>MLEYPIGTPQNLA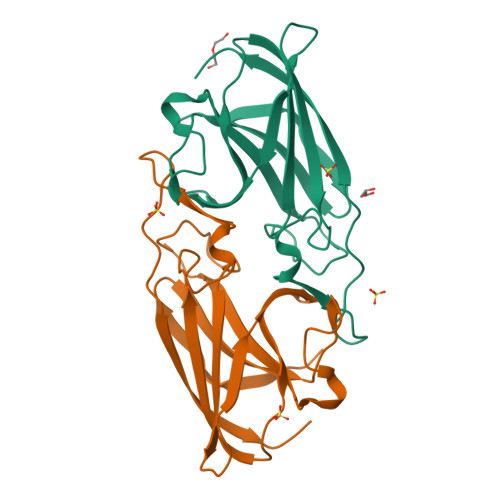GMEIAAVYLQPIDMEPEGHMRKASESDIHIEADIHALSNNPNGYPEGFWVPFLFIKYEITKVGGSGAPITGDMMAMVASDGPHYGDNVKLQGPGKYKVKYTIYPPNAKENPMSPYYGRHTDRETGVRPWFKTFSVEWDFTYAGIGKKGGYAAALEHHHHHH[2x]>[3x]MAKGGFNLSDWALRHQSLVWYLMAVSLVMGVFSYLNLGREEDPSFAIKTMVIQTRWPGATVDDTLEQVTDRIEKKLEELDSLDYVKSYTRPGESTVFVYLKDTTKAGDIPDIWYQVRKKISDIQGEFPQGIQGPGFNDEFGDVFGSVYAFTADGLDFRQLRDYVEKVRLDIRSVKDLGKVQMIGAQNEVIYLNFSTRKLAALGLDQRQVVQSLQAQNAVTPSGVVEAGPERISVRTSGNFRSEKDLQAVNLRVNDRFYRLSDLASISRDFVDPPTSLFRYKGEPAIGLAVAMKEG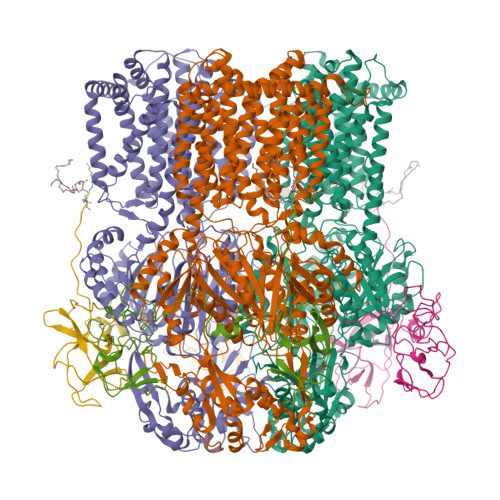GNILEFGEALNARMQEITGELPVGVGVHQVSNQAQVVKKAVGGFTRALFEAVVIVLIVSFVSLGLRAGLVVACSIPLVLAMVFVFMEYTDITMQRVSLGALIIALGLLVDDAMITVEMMITRLELGDSLHDSATYAYTSTAFPMLTGTLVTVAGFVPIGLNASSAGEYTFTLFAVIAVALLLSWIVAVLFAPVIAVHILPKTLKHKSEQKKGRIAERFDSLLHLAMRRRWTTIFLTALLFGVSLFLMKFVQHQFFPSSDRPELLVDLNLPQNSSIHETRAVMDRLEATLKDDEDIDHWSAYVGEGAIRFYLPLDQQLQNNFYGQLVIVTKDLEARERVAARLRDRLRKDYVGISTYVQPLEMGPPVGRPIQYRVSGPQIDKVREYAMGLAGVLDGNPNIGDIVYDWNEPGKMLKIDIAQDKARQLGLSSEDVAQIMNSVVTGSAVTQVRDDIYLVNVIGRAEDSERGSLETLESLQIVTPSGTSIPLKAFAKVSYELEQPLVWRRDRKPTITVKASLRGEIQPTDLVARLAPEVKRFADGLPANYRIEVGGTVEESGKAEGPIAKVVPLMLFLMATFLMIQLQSVQKLFLVASVAPLGLIGVVAALLPTGTPMGFVAILGILALIGIIIRNSVILVTQIDAFEKDGKTPWEAVLEATHHRTRPILLTAAAASLGMIPIAREVFWGPMAYAMIGGIVAATLLTLIFLPALYVAWYRIPEPGRHHHHHH;>CGAEPPAEEHVRVLAQTVKMAEFASATSITGDIQARVQADQSFRVGGKIVERLVDVGDHVAAGQVLARLDPQDQRSNVENAQAAVAAQQAQSKLADLNYQRQKALLPKGYTSQSEYDQALASVRSAQSSLKAAQAQLANARDLLSYTELRASDAGVITARQAEVGQVVQATVPIFTLARDGERDAVFNVYESLFSHDVDGQRITVSLLGKPEVTASGKVREITPTVDERSGTLKVKVGLDSVPAEMSLGSVVNASVAAPAEHSVVLPWSALSKVGEQPAVWLLDQQGKARLQPVRVARYASEKVVIDGGLEAGQTVVTVGGQLLHPGQVVEVAQPPQPTQSTASRDAVGGGQPGNSRGGDEPPPAPPRPVLTVTVKTLKNDDLGRFAGSIQARYESVLGFRTNGRIASRLFDVGDFVGKGALLATLDPTDQQNQLRASQGDLASAEAQLIDAQANARRQEELFARSVTAQARLDDARTRLKTSQASFDQAKAAVQQARDQLSYTRLVTDFDGVITTWHAEAGQVVSAGQAVVTLARPEVREAVFDLPTEVAESLPADARFLVSAQLDPQARTTGSIRELGPQADASTRTRRVRLSLAQTPEAFRLGSTIQVQLSSAGSVRSVLPASVLLERDGKTQVWVVDGKQSSVALREVQVLSRDERQVVIGQGLADGDRVVRAGVNSLKPGQKIKLDEDAR[3x]> DDDDKIVGGYTCGANTVPYQVSLNSGYHFCGGSLINSQWVVSAAHCYKSGIQVRLGEDNINVVEGNEQFISASKSIVHPSYNSNTLNNDIMLIKLKSAASLNSRVASISLPTSCASAGTQCLISGWGNTKSSGTSYPDVLKCLKAPILSDSSCKSAYPGQITSNMFCAG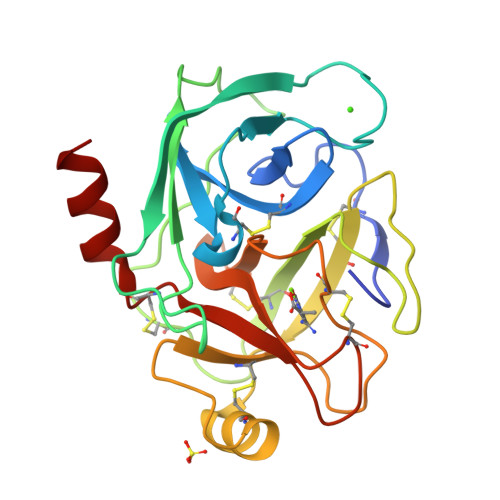YLEGGKDSCQGDSGGPVVCSGKLQGIVSWGSGCAQKNKPGVYTKVCNYVSWIKQTIASN> SGIVQQQNNLLRAIEAQQHLLQLTVWGIKQL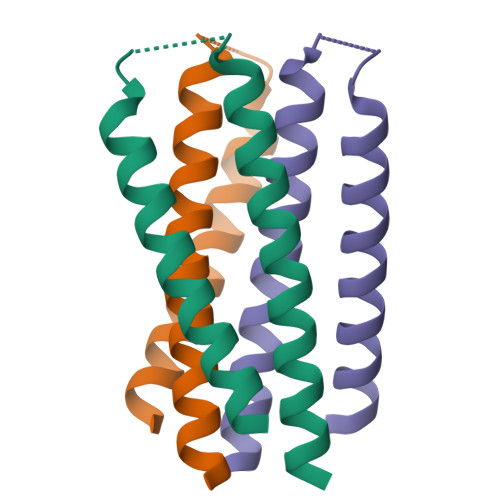QARSGGRGGWMEWDREINNYTSLAHSLIEESQNQQEK>MKTNPLPATPSVWGGSTVELPPTTRDTAGQGLLRRVLRPPISRRDGPVLPRGSGPRRAASTLWLLGLDGTDAPPGALTPNDDTEQALDKILRGTMRGGAALIGSPRHHLTRQVILTDLCQPNADRAGTLLLALRHPADLPHLAHQRAPPGRQTERLGEAWGQLMEATALGSGRAESGCTRAGLVSFNFLVAACAASYDARDAADAVRAHVTANYRGTRVGARLDRFSECLRAMVHTHVFPHEVMRFFGGLVSWVTQDELASVTAVCAGPQEAAHTGHPGRPRSAVILPACAFVDLDAELGLGGPGAAFLYLVFTYRQRRDQELCCVYVIKSQLPPRGLEPALERLFGRLRITNTIHGTEDMTPPAPNRNPDFPLAGLAANPQTPRCSAGQVTNPQFADRLYRWQPDLRGRPTARTCTYAAFAELGMMPEDSPRCLHRTERFGAVSVPVVILEGVVWRPGEWRACA[2x];>MLADGFETDIAIPSGISRPDAAALQRCEGRVVFLPTIRRQLTLADVAHESFVSGGVSPDTLGLLLAYRRRFPAVITRVLPTRIVACPLDVGLTHAGTVNLRNTSPVDLCNGDPISLVPPVFEGQATDVRLDSLDLTLRFPVPLPSPLAREIVARLVARGIRDLNPSPRNPGGLPDLNVLYYNGSRLSLLADVQQLGPVNAELRSLVLNMVYSITEGTTIILTLIPRLFALSAQDGYVNALLQMQSVTREAAQLIHPEAPALMQDGERRLPLYEALVAWLTHAGQLGDTLALAPVVRVCTFDGAAVVRSGDMAPVIRYP[4x];>MIAGTPPHSTMERGGDRDIVVTGARNQFAPDLEPGGSVSCMRSSLSFLSLIFDVGPRDVLSAEAIEGCLVEGGEWTRATAGPGPPRMCSIVELPNFLEYPGARGGLRCVFSRVYGEVGFFGEPAAGLLETQCPAHTFFAGPWALRPLSYTLLTIGPLGMGLFRDGDTAYLFDPHGLPEGTPAFIAKVRAGDMYPYLTYYTRDRPDVRWAGAMVFFVPSGPEPAAPADLTAAALHLYGASETYMQDEAFSERRVAITHPLRGEIAGLGEPCVGVGPREGGGGPGPHPPTAAQSPPPTRARRDDRASETSRGTAGPSAKPEAKRPNRAPDDVWAVALKGTPPTDPPSADPPSAIPPPPPSAPKTPAAEAAEEDDDDMRVLEMGVVPVGRHRARYSAGLPKRRRPTWTPPSSVEDLTSGEKTKRSAPPAKTKKKSTPKGKTPVGAAVPASVPEPVLASAPPDPAGPPVAEAGEDDGPMVPASSQALEALKTRRSPEPPGADLAQLFEAHPNVAATAVKFTACSATLAREVAACSRLTISALRSPYPASPGLLELCVIFFFERVLAFLIENGARTHTQAGVAGPAAALLEFTLSMLPRKTAVGDFLASTRLSLADVAAHLPLVQHVLDENSLIGRLALAKLILVARDVIRETDAFYGELADLELQLRAAPPANLYTRLGEWLLERSQAHPDTLFAPATPTHPEPLLYRVQALAKFARGEEIRVEAEDRQMREALDALARGVDAVSQHAGPLGVMPAPAGAAPQGAPRPPPLGPEAVQVRLEEVRTQARRAIEGAVKEYFYRGAVYSAKALQASDNNDRRFHVASAAVVPVVQLLESLPVFDQHTRDIAQRAAIPAPPPIATSPTAILLRDLIQRGQTLDAPEDLAAWLSVLTDAANQGLIERKPLDELARSIRDINDQQARRSSGLAELRRFDALDAALGQQLDSDAAFVPAPGASPYPDDGGLSPEATRMAEEALRQARAMDAAKLTAELAPDARARLRERARSLEAMLEGARERAKVARDAREKFLHKLQGVLRPLPDFVGLKACPAVLATLRASLPAGWSDLPEAVRGAPPEVTAALRADMWGLLGQYRDALEHPTPDTATALSGLHPSFVVVLKNLFADAPETPFLLQFFADHAPIIAHAVSNAINAGSAAVATADPASTVDAAVRAHRVLVDAVTALGAAASDPASPLAFLAAMADSAAGYVKATRLALDARGAIAQLTTLGSAAADLVVQVRRAANQPEGEHASLIQAATRATTGARESLAGHEGRFGGLLHAEGTAGDHSPSGRALQELGKVIGATRRRADELEAAIADLREKMAAQRARSSHERWAADVEAVLDRVESGAEFDVVELRRLQALAGTHGYNPRDFRKRAEQALGTNAKAVTLALETALAFNPYTPENQRHPMLPPLAAIHRIDWSAAFGAAADTYADMFRVDTEPLARLLRLAGGLLERAQANDGFIDYHEAVLHLSEDLGGVPALRQYVPFFQKGYAEYVDIRDRLDALRADARRAIGSVALDLAAAAEEISAVRNDPAAAAELVRAGVTLPCPSEDALVACVAALERVDQSPVKDTAYADYVAFVTRQDLADTKDAVVRAKQQRAEATERVTAGLREVLAARERRAQLEAEGLANLKTLLKVVAVPATVAKTLDQARSAEEIADQVEILLDQTEKARELDVQAVAWLEHAQRTFETHPLNAASGDGPGLLTRQGARLQALFDTRRRVEALRRSLEEAEAEWDEVWGRFGRVRGGAWKSPEGFRAACEQLRALQDTTNTVSGLRAQRDYERLPAKYQGVLGAKSAERAGAVEELGGRVAQHADLSARLRDEVVPRVAWEMNFDTLGGLLAEFDAVAGDLAPWAVEEFRGARELIQRRMGLYSAYAKATGQTGAGAAAAPAPLLVDLRALDARARASAPPGQEADPQMLRRRGEAYLRVSGGPGPLVLREATSTLDRPFAPSFLVPDGTPLQYALCFPAVTDKLGALLMCPEAACIRPPLPTDTLESASTVTAMYVITVINRLQLALSDAQAANFQLFGRFVRHRQARWGASMDAAAELYVALVATTLTREFGCRWAQLEWGGDAAAPGPPLGPHSSTRHRVSFNENDVLVALVASSPEHIYTFWRLDLVRQHEYMHLTLPRAFQNAADSMLFVQRLTPHPDARIRVLPVFSTGGPPTRGLMFGTRLADWRRGKLSETDPLAPWRSVPELGTERGAALGKLSPAQALAAVSVLGRMCLPSTALAALWTCMFPDDYTEYDSFDALLTARLESGQTLSPSGGREASPPAPPNALYRPTGQHVAVPAAATHRTPAARVTAMDLVLAAVLLGAPVVVALRNTTAFSRESELELCLTLFDSRARGPDAALRDAVSSDIETWAVRLLHADLNPIENACLAAQLPRLSALIAERPLARGPPCLVLVDISMTPVAVLWENPDPPGPPDVRFVGSEATEELPFVAGGEDVLAASATDEDPFLARAILGRPFDASLLSGELFPGHPVYQRAPDDQSPSVPNPTPGPADLVGTEGSLGPGSLAPTLFTDATPGEPVPPRMWAWIHGLEELASDDSGGPAPLLAPDPLSPTADQSVPTSQCAPRPPGPAVTAREARPGVPAESTRPAPVGPRDDFRRLPSPQSSPAPPDATAPRPPASSRASAASSSGSRARRHRRARSLARATQASATTQGWRPPALPDTVAPVTDFARPPAPPKPPEPALHALVSGVPLPLGPQFAGQASPALPIDPVPPPVATGTVLPGGENRRPPLTSGPAPTPPRVPVGGPQRRLTRPAVASLSESRESLPSPWDPADPTAPVLGRNPAEPTSSSPAGPSPPPPAVQPVTPPPTSGPPPTYLTLEGGVTPGGPVSRRPTTRQPVATPTTSARPRGHLTVNRLSAPQPQPQPQPQPQPQPQPQPQPQPQPQPQPQNGHVAPGEYPAVRFRAPQNRPSVPASASSTNPRTGSSLSGVSSWASSLALHIDATPPPVSLLQTLYVSDDEDSDTTSLFLSDSEAEALDPLPREPHSPITNEPFSALSADDSQEVTRLQFGPPPVSANAVLSRRYVQRTGRSALAVLIRACYRLQQQLQRTRRALLHHSDAVLTSLHHVRMLLG[2x];> MNAHLANEVQYDLGHVPGRPSSLVHVIISSECLAAAGIPLAALMRGRPGLGTAANFQVEIQTRAHATGDCTPWCTAFAAYVPADAVGELLAPVVPAHPGLLPRASSAGGLFVSLPVVCDAQGVYDPYAVAALRLAWGSGASCARVILFSYDELVPPNTRYAADSTRIMRVCRHLCRYVALLGAAAPPAAKEAAAHLSMGLGESASPRPQPLARPHAGAPADPPIVGASDPPISPEEQLTAPGGDTTAAQDVSIAQENEEILALVQRAVQDVTRRHPVRARTGRAACGVASGLRQGALVHQAVSGGAMGAADADAVLAGLEPPGGGRFVAPVPHGPGGEDILNDVLTLTPGTAKPRSLVEWLDRGWEALAGGDRPDWLWSRRSISVVLRHHYGTKQRFVVVSYENSVAWGGRRARPPLLSSALATALTEACAAERVVRPHQLSPAGQAELLLRFPALEVPLRHPRPVLPPFDIAAEVAFTARIHLACLRALGQAIRAALQGGPRISQRLRYDFGPDQRAWLGEVTRRFPILLENLMRAVEGTAPDAFFHTAYALAVLAHLGGRGGRGRRVVPLGDDLPARFADSDGHYVFDYYSTSGDTLRLNNRPIAVAMDGDVSKREQSKCRFMEAVPSTAPRRVCEQYLPGESYAYLCLGFNRRLCGI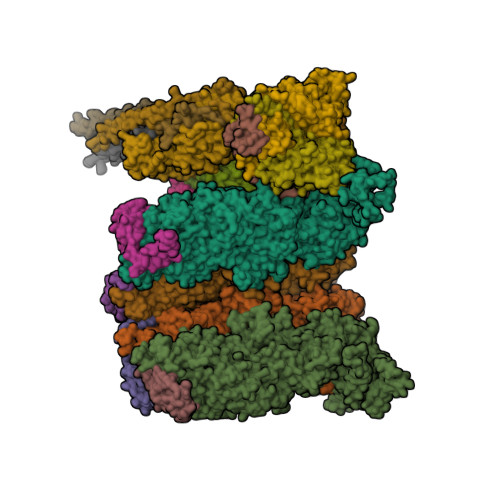VVFPGGFAFTINIAAYLSLSDPVARAAVLRFCRKVSSGNGRSR;>[4x]MAVPQFHRPSTVTTDSVRALGMRGLVLATNNSQFIMDNNHPHPQGTQGAVREFLRGQAAALTDLGLAHANNTFTPQPMFAGDAPAAWLRPAFGLRRTYSPFVVREPSTPGTP;>MDPYCPFDALDVWEHRRFIVADSRNFITPEFPRDFWMSPVFNLPRETAAEQVVVLQAQRTAAAAALENAAMQAAELPVDIERRLRPIERNVHEIAGALEALETAAAAAEEADAARGDEPAGGGDGGAPPGLAVAEMEVQIVRNDPPLRYDTNLPVDLLHMVYAGRGATGSSGVVFGTWYRTIQDRTITDFPLTTRSADFRDGRMSKTFMTALVLSLQSCGRLYVGQRHYSAFECAVLCLYLLYRNTHGAADDSDRAPVTFGDLLGRLPRYLACLAAVIGTEGGRPQYRYRDDKLPKTQFAAGGGRYEHGALASHIVIATLMHHGVLPAAPGDVPRDASTHVNPDGVAHHDDINRAAAAFLSRGHNLFLWEDQTLLRATANTITALGVIQRLLANGNVYADRLNNRLQLGMLIPGAVPSEAIARGASGSDSGAIKSGDNNLEALCANYVLPLYRADPAVELTQLFPGLAALCLDAQAGRPVGSTRRVVDMSSGARQAALVRLTALELINRTRTNPTPVGEVIHAHDALAIQYEQGLGLLAQQARIGLGSNTKRFSAFNVSSDYDMLYFLCLGFIPQYLSAV[2x];>[4x]MAAPNRDPPGYRYAAAMVPTGSLLSTIEVASHRRLFDFFSRVRSDANSLYDVEFDALLGSYCNTLSLVRFLELGLSVACVCTKFPELAYMNEGRVQFEVHQPLIARDGPHPIEQPTHNYMTKIIDRRALNAAFSLATEAIALLTGEALDGTGISAHRQLRAIQQLARNVQAVLGAFERGTADQMLHVLLEKAPPLALLLPMQRYLDNGRLATRVARATLVAELKRSFCETSFFLGKAGHRREAVEAWLVDLTTATQPSVAVPRLTHADTRGRPVDGVLVTTAPIKQRLLQSFLKVEDTEADVPVTYGEMVLNGANLVTALVMGKAVRSLDDVGRHLLEMQEEQLDLNRQTLDELESAPQTTRVRADLVSIGEKLIFLEALEKRIYAATNVPYPLVGAMDLTFVLPLGLFNPVMERFAAHAGDLVPAPGHPDPRAFPPRQLFFWGKDRQVLRLSLEHAIGTVCHPSLMNVDAAVGGLNRDPVEAANPYGAYVAAPAGPAADMQQLFLNAWGQRLAHGRVRWVAEGQMTPEQFMQPDNANLALELHPAFDFFVGVADVELPGGDVPPAGPGEIQATWRVVNGNLPLALCPAAFRDARGLELGVGRHAMAPATIAAVRGAFEDRNYPAVFYLLQAAIHGSEHVFCALARLVVQCITSYWNNTRCAAFVNDYSLVSYVVTYLGGDLPEECMAVYRDLVAHVEALAQLVDDFTLTGPELGGQAQAELNHLMRDPALLPPLVWDCDALMRRAALDRHRDCRVSAGGHDPVYAAACNVATADFNRNDGQLLHNTQARAADAADDRPHRGADWTVHHKIYYYVMVPAFSRGRCCTAGVRFDRVYATLQNMVVPEITPGEDCPSDPVTDPAHPLHPANLVANTVNAMFHNGRVVVDGPAMLTLQVLAHNMAERTTALLCSAAPDAGANTASTTNMRIFDGALHAGILLMAPQHLDHTIQNGDYFYPLPVHALFAGADHVANAPNFPPALRDLSRQVPLVPPALGANYFSSIRQPVVQHVRESAAGENALTYALMAGYFKISPVALHHQLKTGLHPGFGFTVVRQDRFVTENVLFSERASEAYFLGQLQVARHETGGGVNFTLTQPRGNVDLGVGYTAVVATATVRNPVTDMGNLPQNFYLGRGAPPLLDNAAAVYLRNAVVAGNRLGPAQPVPVFGCAQVPRRAGMDHGQDAVCEFIATPVSTDVNYFRRPCNPRGRAAGGVYAGDKEGDVTALMYDHGQSDPSRAFAATANPWASQRFSYGDLLYNGAYHLNGASPVLSPCFKFFTSADIAAKHRCLERLIVETGSAVSTATAASDVQFKRPPGCRELVEDPCGLFQEAYPLTCASDPALLRSARNGEAHARETHFAQYLVYDASPLKGLAL> MAAVSGKSEAAEIEAGDRLDALRDQLQRYETPIIQTILARSALGGRAPSEQDEVRAALSRNAFEPSEVISEWLQTESGARFRSTRPLPPAVEFITPVVLSRDTVLDKPVVGKGIFPIGRRPQDPTNMDEFLDTSLLSLNQSSTVDLASAVSLDVSLLHLVSARVLLGYPIALAKFDWLHDNFCHILTNTTLSKSQKLANIIQQLTDHKQEVNVLSRVEQKSKSLSHLFRNDIPYPPHTQDRILRLFQAYLIPITTQIEAAAILDHANK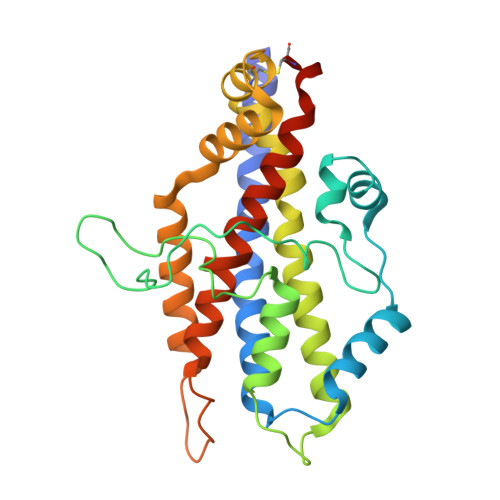CTLEHHHHHH HEPTANYL-P-PHENOL | C13 H20 O | 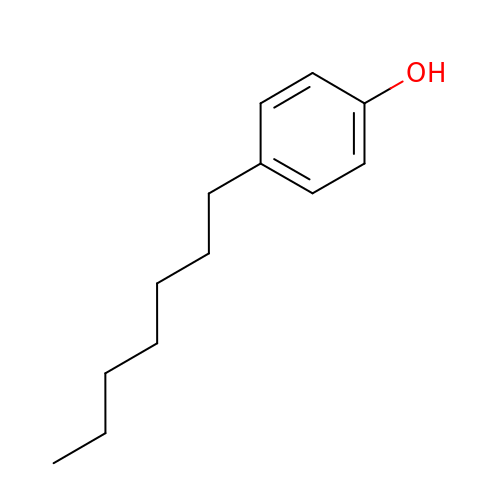KNDDEFBFJLKPFE-UHFFFAOYSA-N> GPVEDAVTAAIGRVADTVGTGPTNSEAIPALTAAETGHTSQVVPGDTMQTRHVKNYHSRSESTVENFLCRSACVYFTEYKNSGSKRYAEWVVTTRQAAQLRRKLEFFTYIRFDLELTFVITSTQQPSTTQNQDAQILTHQIMYVPPGGPVPDKVDSYVWQTST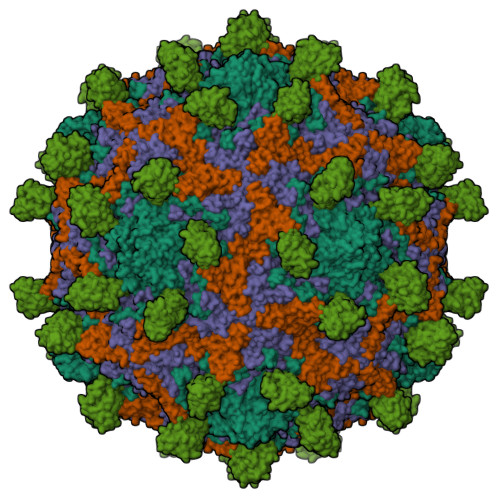NPSVFWTEGNAPPRMSIPFLSIGNAYSNFYDGWSDFSRDGVYGINTLNSMGTLYARHVNTGGTGPIKSTIRIYFKPKHVKAWIPRPPRLCQYEKAKNVNFQPSGVTTTRQSITAMTNTGAF;> SPTVEECGYSDRVRSITLGNSTITTQECANVVVGYGVWPDYLKDNEATAEDQPTQPDVATCRFYTLDSVQWQKTSPGWWWKLPDALSNLGLFGQNMQYHYLGRTGYTIHVQCNASKFHQGCLLVVCVPEAEMGCATLDNTPSSAELLGGDAAKEFAGEPIASGSNKLVQRVVYNAGMGIGVGNLTIFPHQWINLRTNNSATIVMPYTNSVPMDNMFRHNNVTLMVIPFVPLDYCPGSTTYVPITVTIAPMNAEYNGLRLAGHQ;> GLPTMNTPGSCQFLTSDDFQSPSAMPQYDVTPEMRIPGEVKNLMEIAEVDSVVPVQNVGEKVNSMEAYQIPVRSNEGSGTQVFGFPLQPGYSSVFSRTLLGEILNYYTHWSGSIKLTFMFCGSAMATGKFLLAYSPLGAGAPTKRVDAMLGTHVVWDVGLQSSCVLCIPWISQTHYRYVASDECTAGGFITCWYQTNIVVPADAQSSCYIMCFVSACNDFSVRLLKDTPFISQENFFQ;> GAQVSTQKTGAHETGLNASGNSIIHYTNINYYKDAASNSATRQDFAQDPGKFTEPVKDIMIKSLPALN;> MSITTPEEMIEKAKGETAYLPCKFTLSPEDQGPLDIEWLISPADNQKVDQVIILYSGDKIYDDYYPDLKGRVHFTSNDLKSGDASINVTNLQLSDIGTYQCKVKKAPGVANKKIHLVVLVKPSGARCYVDGSEEIGSDFKIKCEPKEGSLPLQYEWQKLSDSQKMPTSWLAEMTSSVISVKNASSEYSGTYSCTVRNRVGSDQCLLRLNVVPPSNKALEHHHHHH>MKKLLPILIGLSLSGFSSLSQAENLMQVYQQARLSNPELRKSAADRDAAFEKINEARSPLLPQLGLGADYTYSNGYRDANGINSNATSASLQLTQSIFDMSKWRALTLQEKAAGIQDVTYQTDQQTLILNTATAYFNVLNAIDVLSYTQAQKEAIYRQLDQTTQRFNVGLVAITDVQNARAQYDTVLANEVTARNNLDNAVEQLRQITGNYYPELAALNVENFKTDKPQPVNALLKEAEKRNLSLLQARLSQDLAREQIRQAQDGHLPTLDLTASTGISDTSYSGSKTRGAAGTQYDDSNMGQNKVGLSFSLPIYQGGMVNSQVKQAQYNFVGASEQLESAHRSVVQTVRSSFNNINASISSINAYKQAVVSAQSSLDAMEAGYSVGTRTIVDVLDATTTLYNAKQELANARYNYLINQLNIKSALGTLNEQDLLALNNALSKPVSTNPENVAPQTPEQNAIADGYAPDSPAPVVQQTSARTTTSNGHNPFRN[3x];>MRYSKLTMLIPCALLLSACTTVTPAYKDNGTRSGPCVEGGPDNVAQQFYDYRILHRSNDITALRPYLSDKLATLLSDASRDNNHRELLTNDPFSSRTTLPDSAHVASASTIPNRDARNIPLRVDLKQGDQGWQDEVLMIQEGQCWVIDDVRYLGGSVHATAGTLRQSIENR[3x]

Tripartite efflux pumps are essential for Gram-negative bacteria to expel a wide range of toxic compounds, including antibiotics, across their dual-membrane cell envelope. Among these systems, the AcrAB–TolC complex of *Escherichia coli* is one of the most thoroughly studied. It comprises the inner membrane RND (Resistance–Nodulation– Division) transporter AcrB, the periplasmic membrane fusion protein AcrA, and the outer membrane channel TolC. Structural analysis reveals that YbjP, a previously uncharacterized lipoprotein, binds TolC in a 3:3 stoichiometry, bridging its protomers at the equatorial domain.

Native purification of *Escherichia coli* membranes yielded a stable assembly containing the outer-membrane channel TolC. Cryo-EM analysis resolved the complex at 3.56 Å resolution ([Fig figs1], [Table tbls1]). The inward-bending HTH coiled-coils occlude the periplasmic tunnel, maintaining TolC in a closed conformation—consistent with previous crystal structures ([Fig fig1]). The YbjP globular domain nestles between adjacent TolC equational domains, forming a stable 3:3 complex ([Fig fig1]). YbjP features a globular domain and a structured N-terminal loop stabilized by a Cys36-Cys144 disulfide bond ([Fig fig1]). The N-terminal loop of YbjP adopts an extended conformation parallel to the first α-helix of TolC’s α-helical barrel, forming substantial intermolecular interfaces. Buried surface area (BSA) analysis reveals 787 Å² of contact with the primary TolC protomer (green in [Fig fig1]), and 1037.4 Å² with the adjacent protomer (light green), suggesting asymmetric binding energetics. The N-terminal density extends to Cys19, which corresponds to the predicted signal peptide cleavage site, positioning the lipoprotein at the periplasmic face of the outer membrane. In the closed state, a complex network of interprotomer hydrogen bonds stabilizes the structure by constricting the pore to its narrowest point at Asp396 ([Fig fig3],[Fig fig3]). In the closed conformation, the coiled-coil helices bundle tightly, leaving a ∼4 Å diameter sealed pore.> AASPAGSHMRLSELASYVSGKLIGEDKEIKVGIFNTLGDANPNDIVIRHWIDEKGVEIAKNKEVSALITQNPKGNSLEYAKKLKVPIILVNKIELASAFAIKWTIKNFAPNTYRVVITGTNGKSTTTHMIYHILT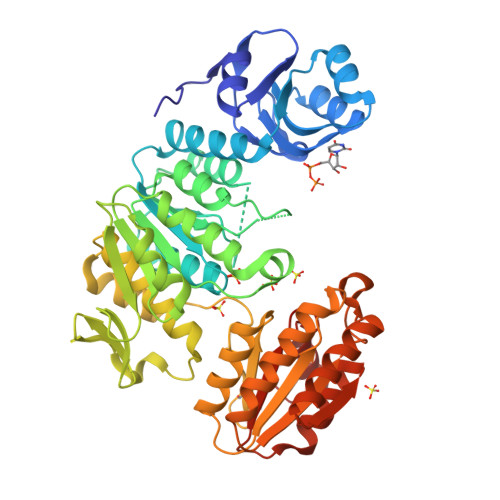HAGKKAFTNTDAKSEFNTLIDPMVAKLLAEKAKKENLEYLVIEVSEVQGWLDRLMKDHAYLMTKSINPNVVVVTNVALDHIGLVNSIEEVFEETSGAVKALEKGFAVLNYDNEFTRKMAKLTNKNVKVFFYGKNCPVTFKSGGIYVNNDLFIKKEELPFKSEYFIQNTLAAISACLCLNIPPDIIKKGILTYKPLKRRFSILCKKPLIIDDFAHNPDGIKMAIKSAKKLTKNKLWVVCAIRGSRGKIINKLNAESLSKTLKNIENYEVVITNSDDVVDNLNKVKKEEEKTFLKTLEKYNINYRFHKKLKTALEETLTNCKKDDTILLIGAQGMDPASKLLKKIKVIPCS>[3x]MQPKLTIWCSEKQVDILQKLGEEFKAKYGVEVEVQYVNFQDIKSKFLTAAPEGQGADIIVGAHDWVGELAVNGLIEPIPNFSDLKNFYETALNAFSYGGKLYGIPYAMEAIALIYNKDYVPEPPKTMDELIEIAKQIDEEFGGEVRGFITSAAE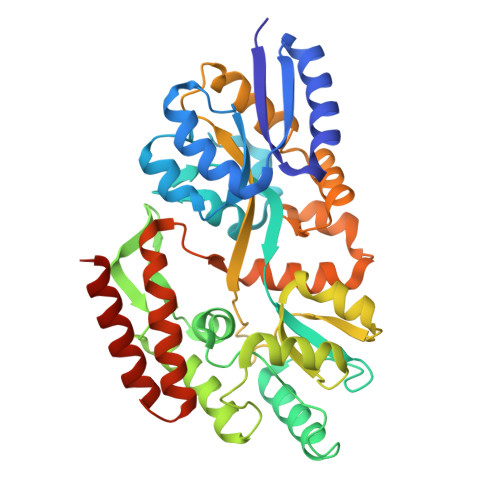FYYIAPFIFGYGGYVFKQTEKGLDVNDIGLANEGAIKGVKLLKRLVDEGILDPSDNYQIMDSMFREGQAAMIINGPWAIKAYKDAGIDYGVAPIPDLEPGVPARPFVGVQGFMVNAKSPNKLLAIEFLTSFIAKKETMYRIYLGDPRLPSRKDVLELVKDNPDVVGFTLSAANGIPMPNVPQMAAVWAAMNDALNLVVNGKATVEEALKNAVERIKAQIQGSHHHHHH> EKLGKLQYSLDYDFQNNQLLVGIIQAAELPALDMGGTSDPYVKVFLLPDKKKKFETKVHRKTLNPVFNEQFTF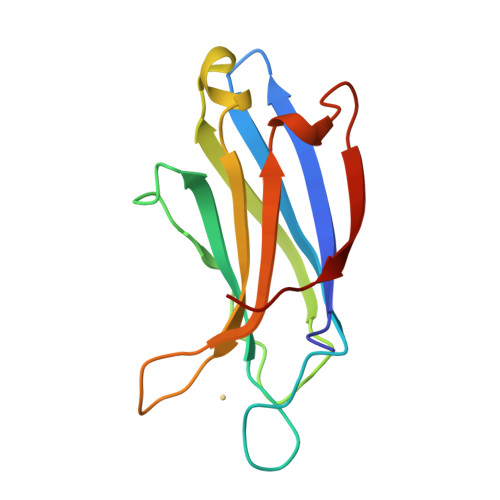KVPYSELGGKTLVMAVYDFDRFSKHDIIGEFKVPMNTVDFGHVTEEWRDLQSA>[2x]MRGSHHHHHHGSACELGPQPMSSQIPSLKDVFLQDFKIGVALPVRVFSNSMDVELITKHFNSMTAENEMKPESILRRDASGKIYYDFTVADRYIEFAQKH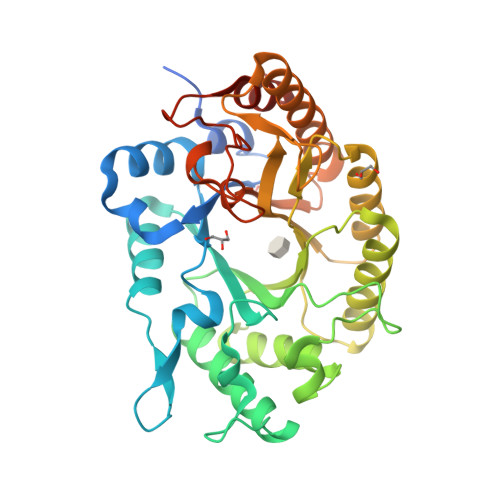GMVVRGHTLVWHSQTPEWFFKDEKGNLLSREAMIERMREYIHTVVGRYRGKVYAWDVVNEAVDENQPDGLRRSLWYQVIGPDYIELAFKFAHEADPDALLFYNDYNEFFPKKRDIIFKLVKEMREKGVPIHGIGMQQHLTLADNVGWIDIAIQKFKTISGIQIHITELDVSVYKSRSPSIIYQTPPSEVLHEQAEFYRKLFEIYRKHTDVITNVTFWGLKDDYSWLRFFFGRRNDWPLLFDENYQPKPAFWSVIESVSKVDLQPSLIS> XQARSDIEKLKEAIRDTNKAVQSVQSSIGNLIVA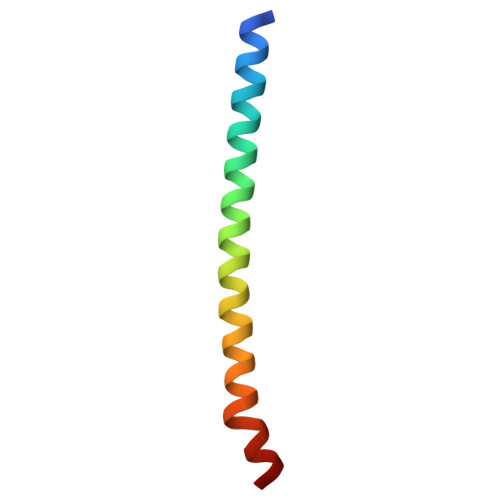IKSVQDYVNKEIVPSIARX>HHHHHHMTDIGAPVTVQVAVDPPYPVVIGTGLLDELEDLLADRHKVAVVHQPGLAETAEEIRKRLAGKGVDAHRIEIPDAEAGKDLPVVG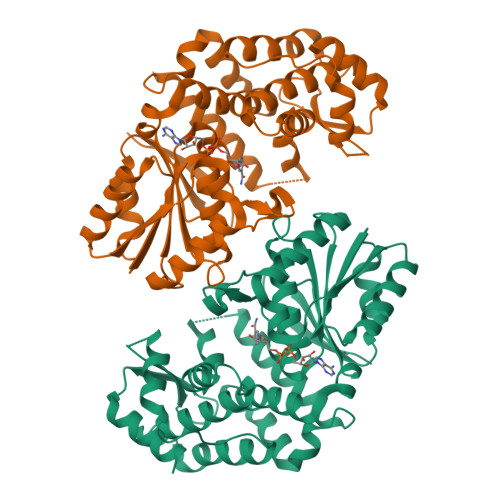FIWEVLGRIGIGRKDALVSLGGGAATDVAGFAAATWLRGVSIVHLPTTLLGMVDAAVGGKTGINTDAGKNLVGAFHQPLAVLVDLATLQTLPRDEMICGMAEVVKAGFIADPVILDLIEADPQAALDPAGDVLPELIRRAITVKAEVVAADEKESELREILNYGHTLGHAIERRERYRWRHGAAVSVGLVFAAELARLAGRLDDATAQRHRTILSSLGLPVSYDPDALPQLLEIMAGDKKTRAGVLRFVVLDGLAKPGRMVGPDPGLLVTAYAGVCAP[2x]> MRGSHHHHHHGRSLNPLSTPQFDSTDETPASYNLAVRRAAPAVVNVYNRGLNTNSHNQLEIRTLGSGVIMDQRGYIITNKHVINDADQIIVALQDGRVFEALLV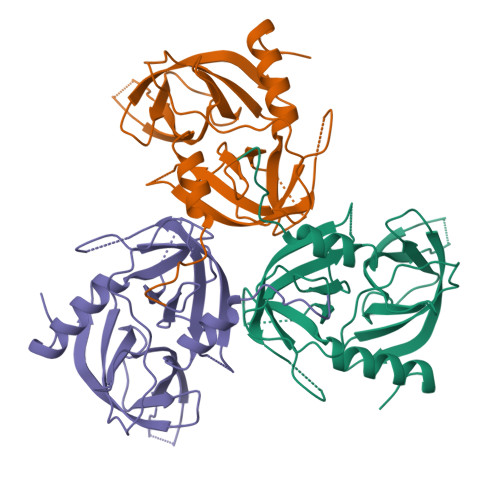GSDSLTDLAVLKINATGGLPTIPINARRVPHIGDVVLAIGNPANLGQTITQGIISATGRIGLNPTGRQNFLQTDASINHGNSGGALVNSLGELMGINTLSFDKSNDGETPEGIGFAIPFQLATKIMDKLIRDGRVIR>[4x]MTNIEPVIIETRLELIGRYLDHLKKFENISLDDYLSSFEQQLITEELLQLITQAAIDINDHILSKLKSGKSYTNFEAFIELGKYQIL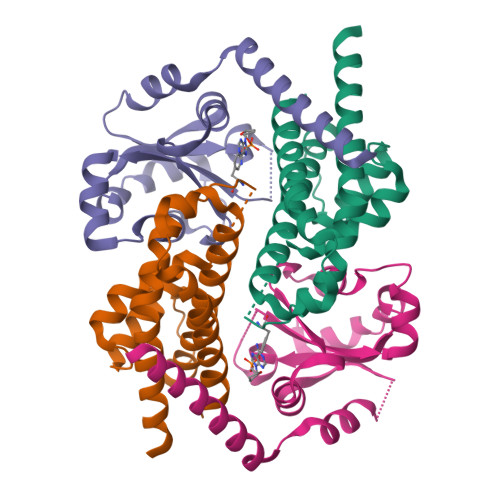TPELAKQIAPSSGLRNRLVHEYDDIDPNQVFMAISFALQQYPLYVRQINSYLITLEEENDLESGHHHHHH;>[4x]MQDKIPTIAELRELSLRLLTKIPYLKMLVLFGSRATGNINANSDWDFAVLYDEEKYNLYIQNNPLAAFVIPGILGEIFKINSDKIDIVELNHCSKLIAHFVARDGKVLYEEPGDEFDKFQQRVLLSNTEIKKIEKTKLENIENFLQRWGV>[4x]SNAMEKFRVIGSTQPLQGEVTISGAKNAALPILFASILAEEPVEVANVPHLRDIDTTMELLERLGAKVERNGSVHVDAGPINQYCAPYDLVKTMRASIWALGPLVARFGQGQVSLPGGCAIGARPVDLHIHGLEQLGATITLEDGYVKAHVDGRLQGAHIVMDKVSVGATITIMCAATLAEGTTVLDNAAREPEIVDTAMFLNKLGAKISGAGTDSITIEGVERLGGGKHAVVPDRIETGTFLVA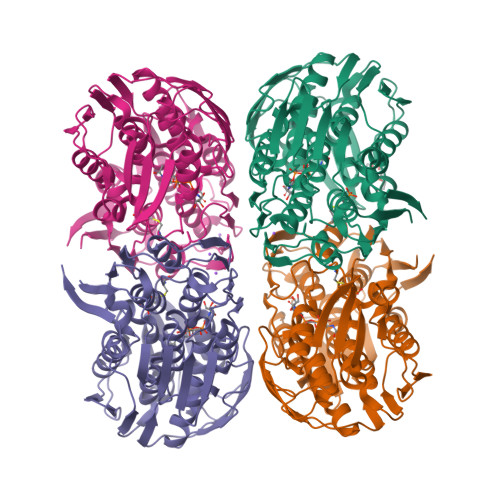AAVSRGKIVCRNTHAHLLEAVLAKLEEAGAEIECGEDWISLDMTGRELKAVTVRTAPHPGFPTDMQAQFTLLNMMAKGGGVITETIFENRFMHVPELKRMGAKAEIEGNTVICGDVDRLSGAQVMATDLRASASLVIAGCIAKGETIVDRIYHIDRGYERIEDKLSALGANIERFRD N-[(1S)-1-(pyridin-3-yl)ethyl]cyclopropanecarboxamide | C11 H14 N2 O | 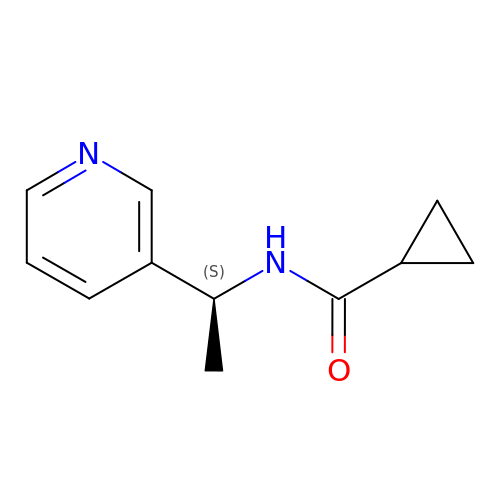XMSIZXIEDPYJDR-QMMMGPOBSA-N> GPALVDADDVMTKEEQIFLLHRAQAQCEKRLKEVLQRPAGRPCLPEWDHILCWPLGAPGEVVAVPCPDYIYDFNHKGHAYRRCDRNGSWELVPGHNRTWANYSECVKFLTNETREREVFDRLGMICTVGYSVSLASLTVAVLILAYFRRLHCTRNYIHMHLFLSFMLRAVSIFVMDAVLYSGATLDEAERLTEEELRAIAQAPPPPATAAAGYAGCRVAVTFFLYFLATNYYWIAVEGLYLHSLIFKAFFSEKKYLWGFTVFGWGLPAIFVAVWVSVRATLANTGCWDLSSGNNKWIIQVPILASIVLNFILFINIVRVLATKGIDCSFWNESYLTGSRDERKKSLLSKFGMDEGVTFMFIGRFDRGQKGVDVLLKAIEILSSKKEFQEMRFIIIGKGDPELE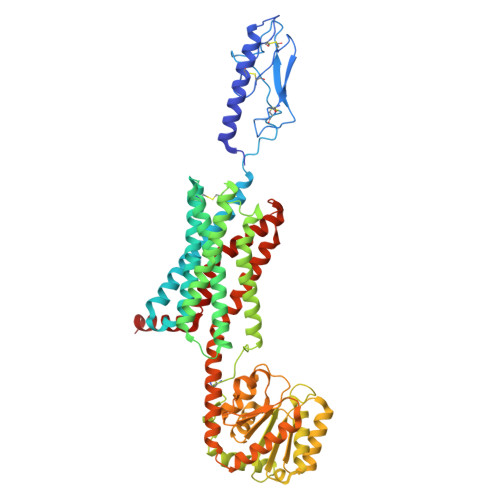GWARSLEEKHGNVKVITEMLSREFVRELYGSVDFVIIPSYFEPFGLVALEAMCLGAIPIASAVGGLRDIITNETGILVKAGDPGELANAILKALELSRSDLSKFRENCKKRAMSFSDTRQQYRKLAKSTLVLMPLFGVHYIVFMLTPYTEVSGTLWQVRMHYEMLFNSFQGFFVAIAYCFCNGEVQAEIKKSWSRWTLA>[10x]MQLVLAAKYIGAGISTIGLLGAGIGIAIVFAALINGVSRNPSIKDTVFPMAILGFALSEATGLFCLMVSFLLLFGV;>ASTKAQPTEVSSILEERIKGVSDEANLNETGRVLAVGDGIARVFGLNNIQAEELVEFSSGVKGMALNLEPGQVGIVLFGSDRLVKEGELVKRTGNIVDVPVGPGLLGRVVDALGNPIDGKGPIDAAGRSRAQVKAPGILPRRSVHEPVQTGLKAVDALVPIGRGQRELIIGDRQTGKTAVALDTILNQKRWNNGSDESKKLYCVYVAVGQKRSTVAQLVQTLEQHDAMKYSIIVAATASEAAPLQYLAPFTAASIGEWFRDNGKHALIVYDDLSKQAVAYRQLSLLLRRPPGREAYPGDVFYLHSRLLERAAKLSEKEGSGSLTALPVIETQGGDVSAYIPTNVISITDGQIFLEAELFYKGIRPAINVGLSVSRVGSAAQVKALKQVAGSLKLFLAQYREVAAFAQFGSDLDASTKQTLVRGERLTQLLKQNQYSPLATEEQVPLIYAGVNGHLDGIELSRIGEFESSFLSYLKSNHNELLTEIREKGELSKELLASLKSATESFVATF[3x];>[3x]ASAAQSTPITGKVTAVIGAIVDVHFEQSELPAILNALEIKTPQGKLVLEVAQHLGENTVRTIAMDGTEGLVRGEKVLDTGGPISVPVGRETLGRIINVIGEPIDERGPIKSKLRKPIHADPPSFAEQSTSAEILETGIKVVDLLAPYARGGKIGLFGGAGVGKTVFIQELINNIAKAHGGFSVFTGVGERTREGNDLYREMKETGVINLEGESKVALVFGQMNEPPGARARVALTGLTIAEYFRDEEGQDVLLFIDNIFRFTQAGSEVSALLGRIPSAVGYQPTLATDMGLLQERITTTKKGSVTSVQAVYVPADDLTDPAPATTFAHLDATTVLSRGISELGIYPAVDPLDSKSRLLDAAVVGQEHYDVASKVQETLQTYKSLQDIIAILGMDELSEQDKLTVERARKIQRFLSQPFAVAEVFTGIPGKLVRLKDTVASFKAVLEGKYDNIPEHAFYMVGGIEDVVAKAEKLAAEAN;> ATLKEVEMRLKSIKNIEKITKTMKIVASTRLSKAEKAKISAKKMDEAEQLFYKNAETKNLDVEATETGAPKELIVAITSDKGLCGSIHSQLAKAVRRHLNDQPNADIVTIGDKIKMQLLRTHPNNIKLSINGIGKDAPTFQESALIADKLLSVMKAGTYPKISIFYNDPVSSLSFEPSEKPIFNAKTIEQSPSFGKFEIDTDANVPRDLFEYTLANQMLTAMAQGYAAEISARRNAMDNASKNAGDMINRYSILYNRTRQAVITNELVDIITGASSLG;> AEAAAASSGLKLQFALPHETLYSGSEVTQVNLPAKSGRIGVLANHVPTVEQLLPGVVEVM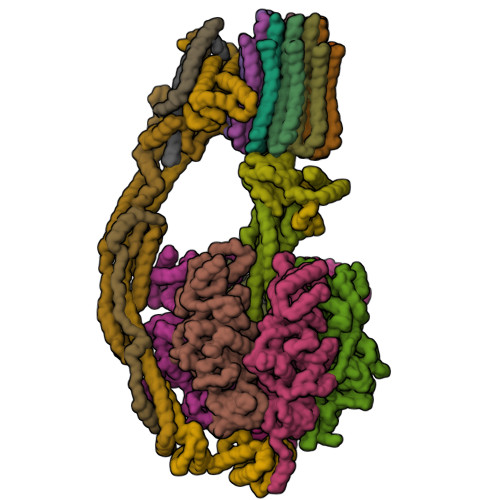EGSNSKKFFISGGFATVQPDSQLCVTAIEAFPLESFSQENIKNLLAEAKKNVSSSDAREAAEAAIQVEVLENLQSVLK;> SAWRKAGISYAAYLNVAAQAIRSSLKTELQTASVLNRSQTDAFYTQYKNGTAASEPTPITK;> ASKAAAPPPVRLFGVEGTYATALYQAAAKNSSIDAAFQSLQKVESTVKKNPKLGHLLLNPALSLKDRNSVIDAIVETHKNLDGYVVNLLKVLSENNRLGCFEKIASDFGVLNDAHNGLLKGTVTSAEPLDPKSFKRIEKALSASKLVGQGKSLKLENVVKPEIKGGLIVELGDKTVDLSISTKIQKLNKVLEDSI;> SPLDQFEIRTLFGLQSSFIDLSCLNLTTFSLYTIIVLLVITSLYTLTNNNNKIIGSRWLISQEAIYDTIMNMTKGQIGGKNWGLYFPMIFTLFMFIFIANLISMIPYSFALSAHLVFIISLSIVIWLGNTILGLYKHGWVFFSLFVPAGTPLPLVPLLVIIETLSYFARAISLGLRLGSNILAGHLLMVILAGLTFNFMLINLFTLVFGFVPLAMILAIMMLEFAIGIIQGYVWAILTASYLKDAVYLH;> NDESILLLTFLGFTGLVAKYLAPAYKDFADARMKKVSDVLNASRNKHVEAVKDRIDSVSQLQNVAETTKVLFDVSKETVELESEAFELKQKVELAHEAKAVLDSWVRYEASLRQLEQRQLAKSVISRVQSELGNPKFQEKVLQQSISEIEQLLSK;> SLAKSAANKLDWAKVISSLRITGSTATQLSSFKKRNDEARRQLLELQSQPTEVDFSHYRSVLKNTSVIDKIESYVKQYKPVKIDASKQLQVIESFEKHAMTNAKETESLVSKELKDLQSTLDNIQSARPFDELTVDDLTKIKPEIDAKVEEMVKKGKWDVPGYKDRFGNLNVM;> VSTLIPPKVVSSKNIGSAPNAKRIANVVHFYKSLPQGPAPAIKANTRLARYKAKYFDGDNASGKPLWHFALGIIAFGYSMEYYFHLRHHKGAEEH;> NVIQDLYLRELKDTKLAPSTLQDAEGNVKPWNPPQKPNLPELELQGPEALKAYTEQNVETAHVAKESEEGESEPIEEDWLVLDDAEETKESH;> MLKRFPTPILKVYWPFFVAGAAVYYGMSKAADLSSNTKEFINDPRNPRFAKGGKFVEVD;> MPQLVPFYFMNQLTYGFLLMITLLILFSQFFLPMILRLYVSRLFISKL N-[oxo(phenylamino)acetyl]-beta-D-glucopyranosylamine 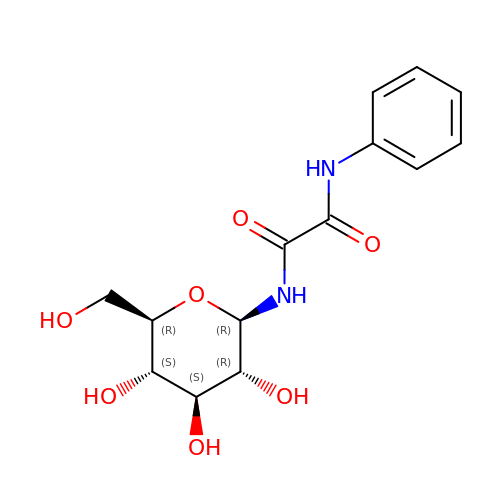| C14 H18 N2 O7 | MWGDULHTYQLGFY-YNXVLUOKSA-N>[4x]EKVIIEKAAGDAEAIAFDGRTYMEYHNAVTKSHLSNEIPAEKALQSNHFELSIKTEATQGLILWSGKGLERS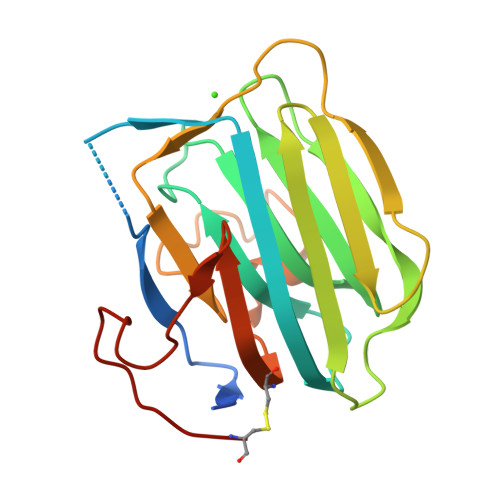DYIALAIVDGFVQMMYDLGSKPVVLRSTVPINTNHWTHIKAYRVQREGSLQVGNEAPITGSSPLGATQLDTDGALWLGGMERLSVAHKLPKAYSTGFIGCIRDVIVDRQELHLVEDALNNPTILHCSAK6-methoxy-7-[3-(piperidin-1-yl)propoxy]quinazolin-4-ol 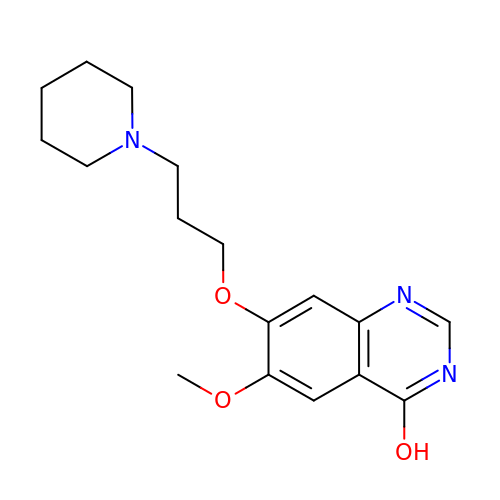| C17 H23 N3 O3 | DMNQXENATQIQBJ-UHFFFAOYSA-N> SIVAPSISIPENQRIPFPKIVGRVVVSDRIPGSKIKLYGKGVDQEPKGIFKINENSGEV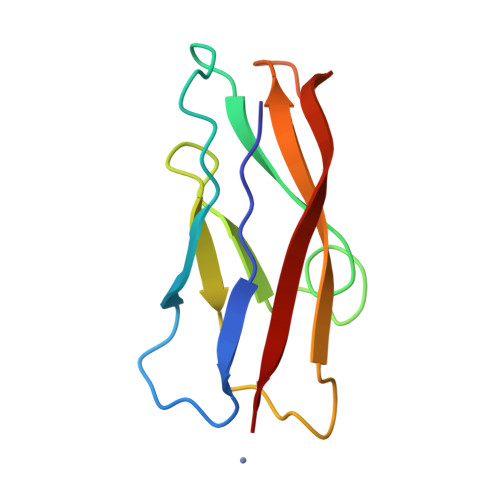SVTKALDREAIPSYQLQVETTDENGKTIEGPVDLEILVID>[2x]ITKSSKSSFSVLDIGLPMSALQRKMMHRLVQYFAFCIDHFCTGPSDSRIQEKIRLFIQSAHNIAKHPSLYDTEVRNPSAAESTNSHVSLDASNFSSYAENSSKFLFLQELFKNLSPSYSKTFFLFISNQFLANTLTQWLKSQNIDAELWAEEDA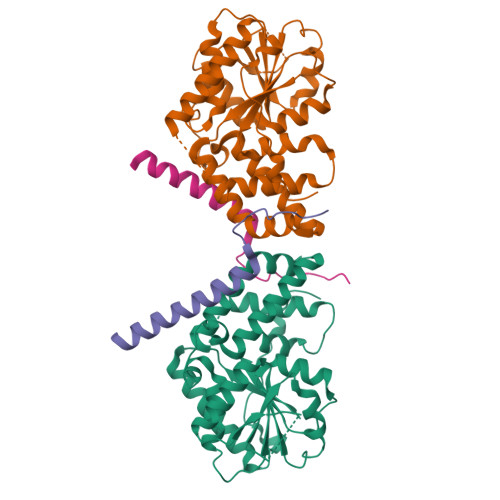KTSQHPAIWICVSKKAPSASHFLQSCPDLSATIFYDIEAYMSVTSSLPSIQSLVLRLIHLGSIEHAIKCFQSSYNASFLVNIVGVVATLSSSSEENSEASNLSTLFEKSGNFEEILGSESHSSITEKTRDIAKNVATWLKNGENFSSWPLPPLMDLASLSVAE;>QIELEYKRKPIPDYDFMKGLETTLQELYVEHQSKKRRLELFQLTN[2x]> MDLTVEPNLHSLITSTTHKWIFVGGKGGVGKTTSSCSIAIQMALSQPNKQFLLISTDPAHNLSDAFGEKFGKDARKVTGMNNLSCMEIDPSAALKDMNDMAVSRANNNGSDGQGDDLGSLLQGGALADLTGSIPGIDEALSFMEVMKHIKRQEQDEGETFDTVIFDTAPTGHTLRFLQLPNTLSKLLEKFGEITNKLGPMLNSFMGAGNVDISGKLNELKANVETIRQQFTDPDLTTFVCVCISEFLSLYETERLIQELISYDMDVNSIIVNQLLFAENDQEHNCKRCQARWKMQKKYLDQIDELYEDFHVVKMPLCAGEIRGLNNLTKFSQFLNKEYNPITDGKVIYELEDKE;> MGSSHHHHHHTNKYHEKWISKFAPGNELSKKYLAKVKERHELKEFNNSISAQDNYAKWTKNN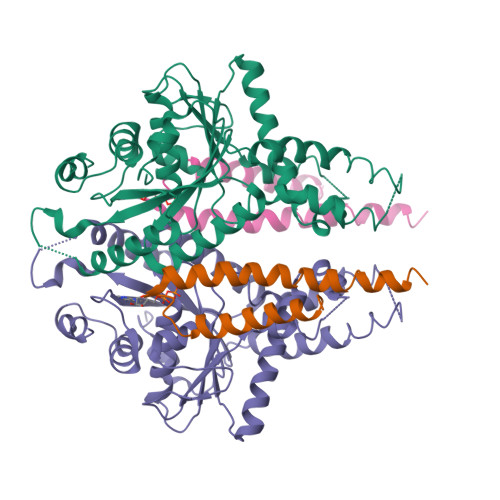RKLDSLDKEINNLKDEIQSENKAFQAHLHKLR>[3x]MKNVGFIGWRGMVGSVLMQRMVEERDFDAIRPVFFSTSQLGQAAPSFGGTTGTLQDAFDLEALKALDIIVTCQGGDYTNEIYPKLRESGWQGYWIDAASSLRMKDDAIIILDPV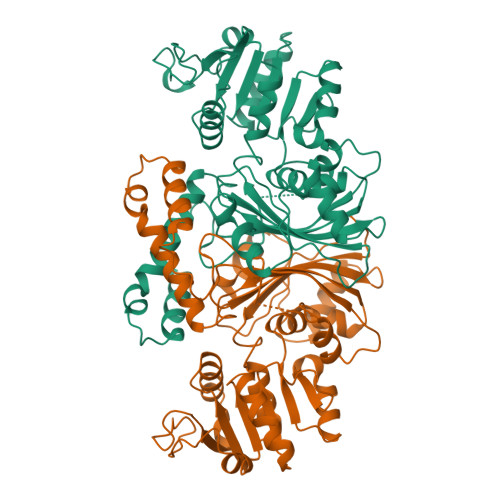NQDVITDGLNNGIRTFVGGNCTVSLMLMSLGGLFANDLVDWVSVATYQAASGGGARHMRELLTQMGHLYGHVADELATPSSAILDIERKVTTLTRSGELPVDNFGVPLAGSLIPWIDKQLDNGQSREEWKGQAETNKILNTSSVIPVDGLCVRVGALRCHSQAFTIKLKKDVSIPTVEELLAAHNPWAKVVPNDREITMRELTPAAVTGTLTTPVGRLRKLNMGPEFLSAFTVGDQLLWGAAEPLRRMLRQLA>MAKRVNTCKCVATPQEKIEYKTKVSRNSNMSKLQAGYLFPEIARRRSAHLLKYPDAQVISLGIGDTTEPIPEVITSAMAKKAHELSTIEGYSGYGAEQGAKPLRAAIAKTFYGGLGIGDDDVFVSDGAKCDISRLQVMFGSNVTIAVQDPSYPAYVDSSVIMGQTGQFNTDVQKYGNIEYMRCTPENGFFPDLSTVGRTDIIFFCSPNNPTGAAATREQLTQLVEFAKKNGSIIVYDSAYAMYMSDDNPRSIFEIPGAEEVAMETASFSNYAGFTGVRLGWTVIPKKLLYSDGFPVAKDFNRIICTCFNGASNISQAGALACLTPEGLEAMHKVIGFYKENTNIIIDTFTSLGYDVYGGKNAPYVWVHFPNQSSWDVFAEILEKTHVVTTPGSGFGPGGEGFVRVSAFGHRENILEACRRF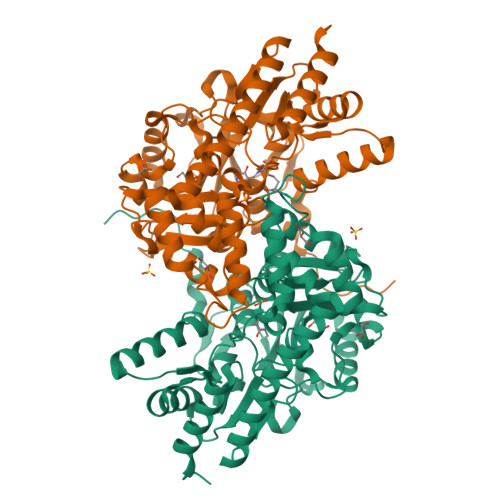KQLYKHHHHHH[2x]>[2x]MWDVIDLSRWQFALTALYHFLFVPLTLGLIFLLAIMETIYVVTGKTIYRDMTRFWGKLFGINFALGVATGLTMEFQFGTNWSFYSNYVGDIFGAPLAMEALMAFFLESTFVGLFFFGWQRLNKYQHLLVTWLVAFGSNLSALWILNANGWMQYPTGAHFDIDTLRMEMTSFSELVFNPVSQVKFVHTVMAGYVTGAMFIMAISAWYLLRGRERNVALRSFAIGSVFGTLAIIGTLQLGDSSAYEVAQVQPVKLAAMEGEWQTEPAPAPFHVVAWPEQDQERNAFALKIPALLGILATHSLDKPVPGLKNLMAETYPRLQRGRMAWLLMQEISQGNREPHVLQAFRGLEGDLGYGMLLSRYAPDMNHVTAAQYQAAMRGAIPQVAPVFWSFRIMVGCGSLLLLVMLIALVQTLRGKIDQHRWVLKMALWSLPLPWIAIEAGWFMTEFGRQPWAIQDILPTYSAHSALTTGQLAFSLIMIVGLYTLFLIAEVYLMQKYARLGPSAMQSEQPTQQQG;>[2x]MFDYETLRFIWWLLIGVILVVFMISDGFDMGIGCLLPLVARNDDERRIVINSVGAHWEGNQVWLILAGGALFAAWPRVYAAAFSGFYVAMILVLCSLFFRPLAFDYRGKIADARWRKMWDAGLVIGSLVPPVVFGIAFGNLLLGVPFAFTPQLRVEYLGSFWQLLTPFPLLCGLLSLGMVILQGGVWLQLKTVGVIHLRSQLATKRAALLVMLCFLLAGYWLWVGIDGFVLLAQDANGPSNPLMKLVAVLPGAWMNNFVESPVLWIFPLLGFFCPLLTVMAIYRGRPGWGFLMASLMQFGVIFTAGITLFPFVMPSSVSPISSLTLWDSTSSQLTLSIMLVIVLIFLPIVLLYTLWSYYKMWGRMTTETLRRNENELY;>[2x]MWYLLWFVGILLMCSLSTLVLVWLDPRLKS

Cytochrome bd quinol:dioxygen oxidases (called bd oxidases for simplicity hereafter) are terminal reductases exclusively found in bacterial and archaeal respiratory chains. They couple quinol oxidation and release of protons to the periplasmic side with proton uptake from the cytoplasmic side to reduce dioxygen to water. Thus, bd oxidases contribute to the generation of a protonmotive force (pmf) by a vectorial charge transfer. The Escherichia coli aerobic respiratory chain contains three terminal oxidases, cytochrome bo3 oxidase, cytochrome bd-I oxidase (bd-I) and cytochrome bd-II oxidase (bd-II).

Here, we present the 3.0 Å resolution structure of E. coli bd-II with bound aurachin D, a specific inhibitor of quinol oxidation by bd oxidases, as obtained by electron cryo-microscopy (cryo-EM). The homo-dimer contains two oxidase hetero-trimers related by twofold symmetry. Each hetero-trimer consists of the three subunits AppB, AppC and AppX of which the small AppX form the major dimer contact between the two hetero-trimers. Within each hetero-trimer, the large subunits AppB and AppC are related by a pseudo-twofold symmetry axis similar as CydA to CydB from bd-I. AppB and AppC share the same fold with nine TM helices that are arranged in two four-helix bundles and a peripheral helix. The heme groups b558, b595, and d are positioned in between the TM helices of AppC and form a triangular arrangement. Heme b558 is coordinated by His186 and Met393 as axial ligands, heme b595 by Glu445 and heme d by His19. AppB features a long hydrophobic patch in a cleft towards the periplasmic space filled with an extended electron density that was perfectly fitted as ubiquinone-8. The Q-loop consists of six small helices (Qα1, P250-E257; Qα2, L292-T297; Qα3, L307-S332; Qα4, P338-R345; Qα5, L351-Y360, and Qα6, A369-A379) that are connected by short loops. An additional density was identified in the cavity of the Q-loop that was modeled as a bound aurachin D molecule. The inhibitor aurachin is bound in a hydrophobic pocket provided by the Q-loop and TM helices 6 and 7 of AppC. Interactions with Phe269, Val271, Leu291, and Leu295 (the latter two from Qα2) stabilize the Q-loop and it is apparently this interaction with aurachin D that allowed for full resolution of the entire Q-loop.One intriguing example is the African swine fever virus, which stands as the sole mammalian-infecting virus encoding a type II topoisomerase. The ORF P1192R encodes a functional Topo II (pP1192R) which is highly conserved across diverse ASFV isolates. Prior extensive structural and biochemical studies have elucidated key aspects of Topo II catalytic mechanisms. These structures have unveiled the inherent architecture of Topo II, which is characterized by two principal heart-shaped functional domains: the ATPase domain, responsible for ATP hydrolysis to fuel the molecular machinery, and the central domain, which interacts with the DNA duplex and contains a catalytic tyrosine residue that cleaves the DNA duplex. As a result, Topo II not only relaxes DNA supercoiling but also disentangles knots and catenates potentially detrimental to cellular function if left unresolved.

The ATPase domain of pP1192R (1-434) was expressed in E. coli BL21(DE3). Owing to the modest resolution of the ATPase domain in the cryo-EM density map, truncated pP1192R ATPase domain (1-434) with either AMPPNP or ADP was crystallized. The crystal structures of the ATPase domain complexed with AMPPNP and ADP yielded high resolutions of 2.3 Å and 2.6 Å, respectively. Both structures contain a protomer within the crystallographic asymmetric unit and these high-resolution crystal structures were employed in the cryo-EM structure construction. The AMPPNP in the structure of ATPase domain partially acts as an inhibitor of pP1192R but lacks specificity.

> MEAFEISDFKEHAKKKSMWAGALNKVTISGLMGVFTEDEDLMALPIHRDHCPALLKIFDEIIVNATDHERACHNKTKKVTYIKISFDKGVFSCENDGPGIPIAKHEQASLIAKRDVYVPEVASCHFLAGTNINKAKDCIKGGTNGVGLKLAMVHSQWAILTTADGAQKYVQHINQRLDIIEPPTITPSREMFTRIELMPVYQELGYAEPLSETEQADLSAWIYLRACQCAAYVGKGTTIYYNDKPCRTGSVMALAKMYTLLSAPNSTIHTATIKADAKPYSLHPLQVAAVVSPKFKKFEHVSVINGVNCVKGEHVTFLKKTINEMVVKKFQQTIKDKNRKTTLRDSCSNIFIVIVGSIPGIEWTGQRKDELSIAENVFKTHYSIPSSFLTSMTKSIVDILLQSISKKDNHKQVDVDKYTRARNAGGKRAQDCMLHHHHHHHH>[2x]HGYIKEPVSRAYMGALEKQTMGWTAAAQKYGSVIDNPQSVEGPKGFPAAGPPDGRIASANGGSGQIDFGLDKQTADHWVKQNIRGGFNTFTWHYTAPHATSKWHYYITK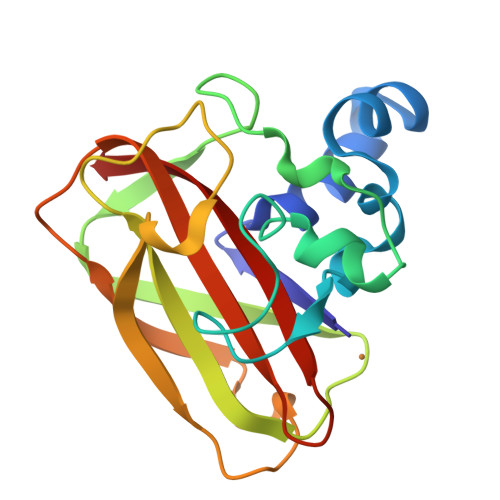KNWNPNKPLSRDEFELIGTVNHDGSKADTNLTHKIFVPTDRSGYHIILGVWDVADTSNAFYNVIDVNLT> MTESNEVLFGIASHFALEGAVTGIEPYGDGHINTTYLVTTDGPRYILQQMNTSIFPDTVNLMRNVELVTSTLKAQGKETLDIVPTTSGATWAEIDGGAWRVYKFIEHTVSYNLVPNPDVFREAGSAFGDFQNFLSEFDASQLTETIAHFHDTPHRFEDFKAALAADKLGRAAACQPEIDFYLSHADQYAVVMDGLRDGSIP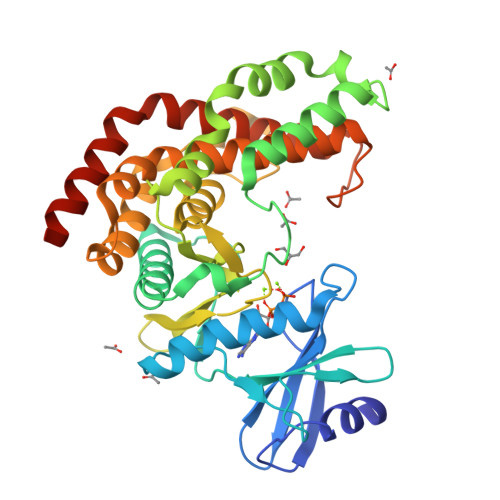LRVTHNDTKLNNILMDATTGKARAIIDLDTIMPGSMLFDFGDSIRFGASTALEDEKDLSKVHFSTELFRAYTEGFVGELRGSITAREAELLPFSGNLLTMECGMRFLADYLEGDIYFATKYPEHNLVRTRTQIKLVQEMEQKASETRAIVADIMEAARLEHHHHHH>[2x]DRDRLRPPLDERSLRDQLIGAGSGWRQLDVVAQTGSTNADLLARAASGADIDGVVLIAEHQTAGRGRHGRGWAATARAQIILSVGVRVVDVPVQAWGWLSLAAGLAVLDSVA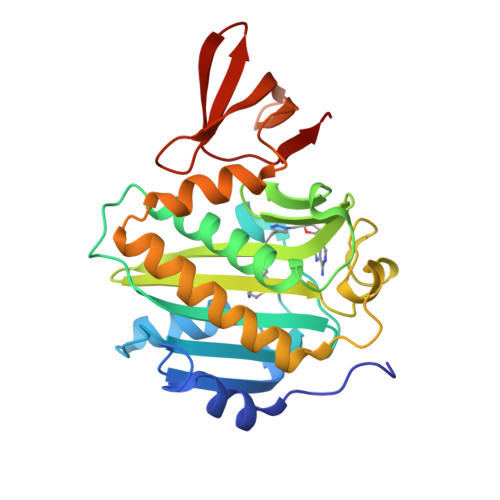PLIAVPPAETGLKWPNDVLARGGKLAGILAEVAQPFVVLGVGLNVTQAPEEVDPDATSLLDLGVAAPDRNRIASRLLRELEARIIQWRNANPQLAADYRARSLTIGSRVRVELPGGQDVVGIARDIDDQGRLCLDVGGRTVVVSAGDVVHLR> MSQNNTISSMNPERAYNNVTLKNLTAFQLLSQRENICELLNLVESTERHNSIINPERQRMSLEEMKKMLDALKNERKK;> MSGSNMGYYDVLAGLSALEKSSQVVFSATELQQLTQQSHATDKGIEGSENSKAKVSKPKRVAVHGYLGGKVSLADAAQVEYEVGHSLLGSYVPRQQLEALSSVDFSHHFHRTLECKAALETHDVFLAGAGQLSLPFQSHIESPRNSEAKRKRKVIICKRCQSRFIGSHRRSQLREHACVD;> MSDSEGGLASEVEHEKRSRSTSNRPNYAIDTEDLDIDENDENEDDDYREEEANEGVNEEEISDEEEQINKSGRNKRRHVDEEEDLSEDKGVTRSRNRSKFKKPVFPGIDDAEENLNPLKVVNEEYVLPDDPEGETKITADGDLLGGREFLVRTFTLTEKGNRKFMLATEPARIVGFRDSYLFFQTHPNLYKFILNQTQKNDLIDRGVLPYSYRNRQIALVTARGVFKEFGAKIIRGGKHITDDYYASELRTKGNVIEGKLAGDPIDKSARALETMMYPASENGINPAKNQVEFFEHRPHGHMSNSNIIASGSKLSSTNWLYQHSAACSRFNSDLFYDRVKVLLVDQQGLRDAYTNILHIPESTQSTTVLGWRRSKNDSPSDTSIVYETVIHDNDLNKPKTGLSEIPKEIYEDVVDEDVLRAITEQQNFEKCNEYI;> MMPDDNSNSSTQNSSALYKDLRKEYESLFTLKEDSGLEISPIFNVLPPKKDYPDYYAVIKNPVSFNTLKKRIPHYTDAQQFMNDVVQIPWNAKTYNTRDSGIYKYALVLEKYLKDTIYPNLKEKYPQLVYPDLGPLPDEPGYEEFQQKLREKAEEVARANAARAESSSSMNSTEAARRLRKTRTSVKRESEPGTDTNNDEDYEATDMDIDNPKDADFPDLIRKPLININPYTRKPLRDNRSTTPSHSGTPQPLGPRHRQVSRTQVKRGRPPIIDLPYIQRMKNVMKVLKKEVLDSGIGLTDLFERLPDRHRDANYYIMIANPISLQDINKKVKTRRYKTFQEFQNDFNLMLTNFRISHRGDPESIKISNILEKTFTSLARFELSKPDRSFIPEGELRYPLDEVIVNNISYHVGDWALLRNQNDPQKPIVGQIFRLWKTPDGKQWLNACWYYRPEQTVHRVDRLFYKNEVMKTGQYRDHLVSNLVGKCYVIHFTRYQRGNPDMKLEGPLFVCEFRYNESDKIFNKIRTWKACLPEEIRDLDEATIPVNGRKFFKYPSPIRHLLPANATPHDRVPEPTMGSPDAPPLVGAVYMRPKMQRDDLGEYATSDDCPRYIIRPNDSPEEGQVDIETGTITTNTPTANALPKTGYSSSKLSSLRYNRSSMSLENQNAIGQQQIPLSRVGSP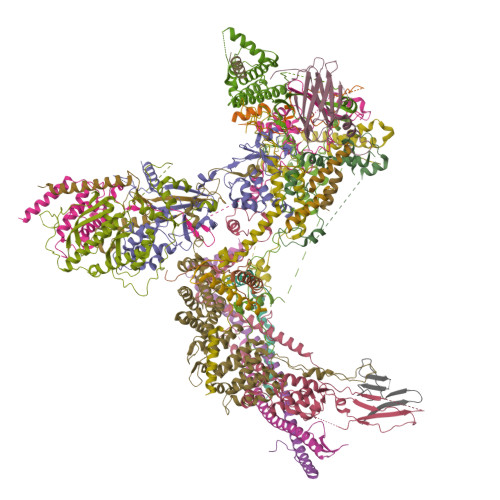GAGGPLTVQGLKQHQLQRLQQQQHQYQQQKRSQASRYNIPTIIDDLTSQASRGNLGNIMIDAASSFVLPISITKNVDVLQRTDLHSQTKRSGREEMFPWKKTKGEILWFRGPSVIVNERIINSGDPHLSLPLNRWFTTNKKRKLEYEEVEETMEDVTGKDKDDDGLEPDVENEKESLPGPFVLGLRPSAKFTAHRLSMLRPPSSSS;> MDIRGRKMKKPPACVQCRKRKIGCDRVKPICGNCMKHNKMDCFYPDVPGQYVPSSSSSSNTRQVANGPYLNSYYASRRVSKETAALLQKNPELASLEQIREYNTRLQLLNAQNQLNNRSSAANATLNQQHTQYIPKSVPSLESKPVTSANESSTPLNWVQGPAIFHMLTSPYTQDEIINHEMNFLKGRLLELQEITGKKITGVNLDLKQDSSAQMQSSHSNRNQEEFLTIKKRKLSEDGVTDGDGKPIPESERRPHLNEFKDLDPQFLDTNKVFNVFNSAISEEGRNRLWLLPKNINKSSIFQIQYLIERDPFLFKFFNDLNILIETQFNGPLHDLVASRNSIERNSGISQILKFPSQSITQTLINKYLSTITETNSILPILKPKRLLPIVEQLFPSNTINKPNSKDFETIFQVFSVTNDQLLNLGFITLCLLILFESLNSTVLIPLRDDEHLQLFNVLFNYLPLLKSNLTTLRFEIEKRSMCNIETLRFISLWKYYQFVMDTSSSSSFVIDYDEDMHMACLLSLNHETQNQSHILTWNFIFKNYCWRHLFLGQLPLLMSEPFTNSTPIIDPLLNNDFELIDFEVNLMKYLQSKDQQLSIDKIIQLIKLLKNKNIEVSQGCLTTPSIINNIMDSLIYRNSMLYLNFYLLLQFETLKNYAKFNEILEDFLELSRETLFFVFSNLANIKFAGHEFTFINKSIVVLQTLVLMLLALYQRSFDSSKRTNDANEISEQTDIHSNNDNSKRIKNKNVIHLIINKIAMLLSDYSKNCKKQNKLIENLIIKIKTISKYIKNLEENKVTTSADSNYSINNGFSGISAEQLIKLNHELSKISESLIKTDFYEQRKNSTVSNGVLGAAAPVDSDANSDTFGLTKENFNEVFEAIRS;> MVVKKRKLATEAGGSDERPKYLPGKHPKNQEKTPHVDYNAPLNPKSELFLDDWHIPKFNRFISFTLDVLIDKYKDIFKDFIKLPSRKFHPQYYYKIQQPMSINEIKSRDYEYEDGPSNFLLDVELLTKNCQAYNEYDSLIVKNSMQVVMLIEFEVLKAKNLKRNYLINSEVKAKLLHYLNKLVDATEKKINQALLGASSPKNLDDKVKLSEPFMELVDKDELPEYYEIVHSPMALSIVKQNLEIGQYSKIYDFIIDMLLVFQNAHIFNDPSALIYKDATTLTNYFNYLIQKEFFPELQDLNERGEINLEFDKFEFENYLAIGGGGPAAAGALAISALDNDIEPESNREDLIDQADYDFNHFEGLGNGYNRSLLTEDYLLNPNNFKKLIAKPETVQSEVKNERSTTSDIEKTNSLESEHLKIPKYNVIKSMQKEMQSLSEQHTMEYKPYKLIQQIYIFSSKNLYSQATKPLLGSRPSCNQNWVEYIFNGNELSQNENAFSFMLQPMQTFLTLQSHLTSSLKDTETLLTINKEPVKSRTSNVNSNLSQPQQQENDVIGNDTKQDIENLTIGGGNNNDIVGNDNDKRNNITEIFDIRLSEGLNHLMFRCEDKISHETEFMNFWINVLP;>[4x]MSDTEKDKDVPMVDSHEATEEPPTTSTNTPSFPHLAQEQAKEESATLGAEVAHKKINYEQEAQKLEEKALRFLAKQTHPVIIPSFASWFDISKIHEIEKRSNPDFFNDSSRFKTPKAYKDTRNFIINTYRLSPYEYLTITAVRRNVAMDVASIVKIHAFLEKWGLINYQIDPRTKPSLIGPSFTGHFQVVLDTPQGLKPFLPENVIKQEVEGGDGAEPQVKKEFPVNLTIKKNVYDSAQDFNALQDESRNSRQIHKVYICHTCGNESINVRYHNLRARDTNLCSRCFQEGHFGANFQSSDFIRLENNGNSVKKNWSDQEMLLLLEGIEMYEDQWEKIADHVGGHKRVEDCIEKFLSLPIEDNYIREVVGSTLNGKGGDSRDGSVSGSKLMECVNDAVQTLLQGDDKLGKVSDKSREISEKYIEESQAIIQELVKLTMEKLESKFTKLCDLETQLEMEKLKYVKESEKMLNDRLSLSKQILDLNKSLEELNVSKKLVLISEQVDSGIQLVEKDQEGDDEDGNTATGHGVKRVGKEGEEVGEGDSIAKLQPQVYKPWSL;> MVTQTNPVPVTYPTDAYIPTYLPDDKVSNLADLKKLIEMDSRLDLYLTRRRLDTSINLPTNTKTKDHPPNKEMLRIYVYNTTESSPRSDSGTPADSGKTTWTLRIEGKLLHESANGKHPFSEFLEGVAVDFKRLKPLGMGKKRKRDSSLSLPLNLQQPEYNDQDSTMGDNDNGEDEDSAEAESREEIVDALEWNYDENNVVEFDGIDIKRQGKDNLRCSITIQLRGVDGGKVQYSPNLATLIGMQTGSVNDAVYSIYKYILINNLFVTEQTEAQDGSNDAEDSSNENNNKNGAGDDDGVEGSTPKDKPELGEVKLDSLLQKVLDTNAAHLPLMNVVQTVNKLVSPLPPIILDYTIDLSKDTTYGATTLDVDVSHILHQPQPQPNLQKEEETDAEDTAKLREITKLALQLNSSAQKYQFFHELSLHPRETLTHYLWSSKQNELVLQGDQYFNEDAARTSDIYSNNNNDRSLMGNISLLYSQGRL;> MNSLASNTPLNGTPVSEAPATSSEPVNMFETMVANPIKVSRLQSNGVLTGPAANTKSIHYSLANFNVFQSLPKETARGVDDLTRMEMALLSGIPEEIKWSLKKYLTYSNKAPYMISLRTLPDLLPLFKTFILPLERIVEGLNKSSICDSKAMDSLQMGLNALLILRNLAQDTDSVQILVKDREIKSFILFILKKFQCVATGDNKWQLYEGNATFFNELTHYTLDLMEAISSYIAPAMKDDHYFQTLVSILNYTKDRYMVISILRSLSRLLVRSKANEESAADNLDHKTLSLIVSFLLLECDSELIIASLDFLYQYILPGSQRITELFKSKECSLILEATLPNLLSYNIATPDYHLLQKHKIRLIKRLKPPAPKEPPNLSEDLFQQLFKLNEPLRSTAWLRCCFEPVQEAEFTQISLWRSYESKFGQPVRESGRKLLPAVEFIKNVSNAFNNAAAIVITDPVTGKKRFVIKGIQPRFKALGIADGERESQVPISALKSKFLNDSKEITPARQNSIPEVKFPQELSDVSKVACTFLCLLSNDTDDGAGSAFCQRIRPLVLHKLADIPPLTLALSEYMENTSGL;> MTESVGGNKLVDFLVNVQSILNAASVKCHVVDESFPAKFFEKNPDKIYESYCKFIKNRSNSEGLIRNEDKLVLTTINKRFENGEYEPIQGGFYKLYHDIKLVCTILIHFYPQGTRNYQLVDKFYKFSSELLLRECCRIGIALTQTNNIKSRSGKLLSGNEMDEYDDDDATELDKIISYDFIKISMNYTVPISQTYQIRTKDMDLFSSIISKSNLDKRPHELPNTNFKINNVLPQTDIENEAPRLGFVGANTSNIPDPTLPPTEMMTRFLHPNWYALPTTVWLKYGNYNSWAPSFNENGTVVDSTTRGLIWLERIGYMDLYEKNEKKVKQEELLNTNEEGINRKQNDENNKNVDGKSNGVQDDGGDNDNDATIASANSESTENKEQFIIKLQNLYNWTPSNYIGDDEIENFRNGTPDKLVSDSLLKLKRLRKERILNKVLKPTTEERELYFKVKRILKEVILAKKVSKVPINNVRAFPVLQTNYNGSIPVVRAQPGRKRKHKK;> MSHQNQLIPQAYISNFHNRLTNEDDGIPIFTMAQQTRQHKRAKVVNYAEYDNDLFDEFNMNGSNFNNADTHYKDNAVSHENTPALTNGVTMDGSEYNVLENMNGADSIISNNKYDAGSNMVVESLSGLNSNNNASNGPSNKAQAQDIGNAVLPDLQDQHHNPFNILRYPKIRDTFINGKVVSPYRLNTDQETKANANSGEAIMIPITLDIEHMGHTIKDQFLWNYNDDSISPEEFASIYCKDLDMTSATLQTQIANIIKEQLKDLENIAATEIMSDLHVIINLTCNLQDRFFEDNFQWNLNDKSLTPERFATSIVQDLGLTREFIPLISQSLHETILKIKKDWVDGHLIQDHVPNDAAFGYLSGIRLDIDELGSNWCPRVEILTKEEIQKREIEKERNLRRLKRETDRLSRRGRRRLDDLETTMRM;> MLQEQSELMSTVMNNTPTTVAALAAVAAASETNGKLGSEEQPEITIPKPRSSAQLEQLLYRYRAIQNHPKENKLEIKAIEDTFRNISRDQDIYETKLDTLRKSIDKGFQYDEDLLNKHLVALQLLEKDTDVPDYFLDLPDTKNDNTTAIEVDYSEKKPIKISADFNAKAKSLGLESKFSNATKTALGDPDTEIRISARISNRINELERLPANLGTYSLDDCLEFITKDDLSSRMDTFKIKALVELKSLKLLTKQKSIRQKLINNVASQAHHNIPYLRDSPFTAAAQRSVQIRSKVIVPQTVRLAEELERQQLLEKRKKERNLHLQKINSIIDFIKERQSEQWSRQERCFQFGRLGASLHNQMEKDEQKRIERTAKQRLAALKSNDEEAYLKLLDQTKDTRITQLLRQTNSFLDSLSEAVRAQQNEAKILHGEEVQPITDEEREKTDYYEVAHRIKEKIDKQPSILVGGTLKEYQLRGLEWMVSLYNNHLNGILADEMGLGKTIQSISLITYLYEVKKDIGPFLVIVPLSTITNWTLEFEKWAPSLNTIIYKGTPNQRHSLQHQIRVGNFDVLLTTYEYIIKDKSLLSKHDWAHMIIDEGHRMKNAQSKLSFTISHYYRTRNRLILTGTPLQNNLPELWALLNFVLPKIFNSAKTFEDWFNTPFANTGTQEKLELTEEETLLIIRRLHKVLRPFLLRRLKKEVEKDLPDKVEKVIKCKLSGLQQQLYQQMLKHNALFVGAGTEGATKGGIKGLNNKIMQLRKICNHPFVFDEVEGVVNPSRGNSDLLFRVAGKFELLDRVLPKFKASGHRVLMFFQMTQVMDIMEDFLRMKDLKYMRLDGSTKTEERTEMLNAFNAPDSDYFCFLLSTRAGGLGLNLQTADTVIIFDTDWNPHQDLQAQDRAHRIGQKNEVRILRLITTDSVEEVILERAMQKLDIDGKVIQAGKFDNKSTAEEQEAFLRRLIESETNRDDDDKAELDDDELNDTLARSADEKILFDKIDKERMNQERADAKAQGLRVPPPRLIQLDELPKVFREDIEEHFKKEDSEPLGRIRQKKRVYYDDGLTEEQFLEAVEDDNMSLEDAIKKRREARERRRLRQNGTKENEIETLENTPEASETSLIENNSFTAAVDEETNADKETTASRSKRRSSRKKRTISIVTAEDKENTQEESTSQENGGAKVEEEVKSSSVEIINGSESKKKKPKLTVKIKLNKTTVLENNDGKRAEEKPESKSPAKKTAAKKTKTKSKSLGIFPTVEKLVEEMREQLDEVDSHPRTSIFEKLPSKRDYPDYFKVIEKPMAIDIILKNCKNGTYKTLEEVRQALQTMFENARFYNEEGSWVYVDADKLNEFTDEWFKEHSS;> MMDMQVRKVRKPPACTQCRKRKIGCDRAKPICGNCVKYNKPDCFYPDGPGKMVAVPSASGMSTHGNGQGSNHFSQGNGVNQKNVMIQTQYPIMQTSIEAFNFSFNPSVDTAMQWTKAASYQNNNTNNNTAPRQNSSTVSSNVHGNTIVRSDSPDVPSMDQIREYNTRLQLVNAQSFDYTDNPYSFNVGINQDSAVFDLMTSPFTQEEVLIKEIDFLKNKLLDLQSLQLKSLKEKSNLNADNTTANKINKTGENSKKGKVDGKRAGFDHQTSRTSQSSQKYFTALTITDVQSLVQVKPLKDTPNYLFTKNFIIFRDHYLFKFYNILHDICHINQFKVSPPNNKNHQQYMEVCKVNFPPKAIIIETLNSESLNNLNIEEFLPIFDKTLLLEFVHNSFPNGDTCPSFSTVDLPLSQLTKLGELTVLLLLLNDSMTLFNKQAINNHVSALMNNLRLIRSQITLINLEYYDQETIKFIAITKFYESLYMHDDHKSSLDEDLSCLLSFQIKDFKLFHFLKKMYYSRHSLLGQSSFMVPAAENLSPIPASIDTNDIPLIANDLKLLETQAKLINILQGVPFYLPVNLTKIESLLETLTMGVSNTVDLYFHDNEVRKEWKDTLNFINTIVYTNFFLFVQNESSLSMAVQHSSNNNKTSNSERCAKDLMKIISNMHIFYSITFNFIFPIKSIKSFSSGNNRFHSNGKEFLFANHFIEILQNFIAITFAIFQRCEVILYDEFYKNLSNEEINVQLLLIHDKILEILKKIEIIVSFLRDEMNSNGSFKSIKGFNKVLNLIKYMLRFSKKKQNFARNSDNNNVTDYSQSAKNKNVLLKFPVSELNRIYLKFKEISDFLMEREVVQRSIIIDKDLESDNLGITTANFNDFYDAFYN> MDPYYPFDALDVWEHRRFIVADSRSFITPEFPRDFYMSPVFNIPRETAAERAAVLQAQRTAAAAALENAALQAAELPVDIERRIRPIEQQVHHIADALEALETAATAAEEADAARDAEARGEGAADGAAPSPTAGPAAAEMEVQIVRNDPPLRYDTNLPVDLLHMVYAGRGAAGSSGVVFGTWYRTIQERTIADFPLTTRSADFRDGRMSKTFMTALVLSLQSCGRLYVGQRHYSAFECAVLCLYLLYRTTHESSPDRDRAPVAFGDLLARLPRYLARLAAVIGDESGRPQYRYRDDKLPKAQFAAAGGRYEHGALATHVVIATLVRHGVLPAA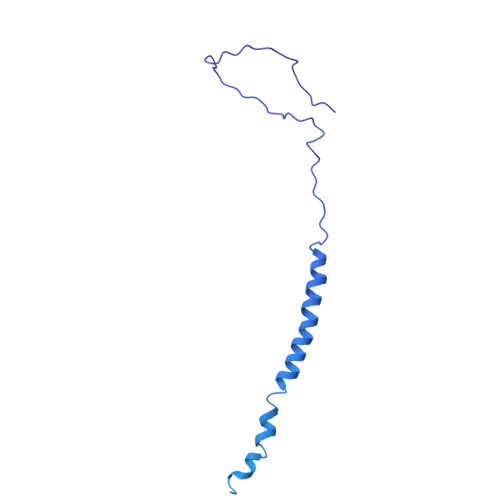PGDVPRDTSTRVNPDDVAHRDDVNRAAAAFLARGHNLFLWEDQTLLRATANTITALAVLRRLLANGNVYADRLDNRLQLGMLIPGAVPAEAIARGASGLDSGAIKSGDNNLEALCVNYVLPLYQADPTVELTQLFPGLAALCLDAQAGRPLASTRRVVDMSSGARQAALVRLTALELINRTRTNTTPVGEIINAHDALGIQYEQGLGLLAQQARIGLASNAKRFATFNVGSDYDLLYFLCLGFIPQYLSVA> MSSDLAAELGFDPALKKKKKTKKVIPDDFDAAVNGKENGSGDDLFAGLKKKKKKSKSVSADAEAEKEPTDDIAEALGELSLKKKKKKTKDSSVDAFEKELAKAGLDNVDAESKEGTPSANSSIQQEVGLPYSELLSRFFNILRTNNPELAGDRSGPKFRIPPPVCLRDGKKTIFSNIQDIAEKLHRSPEHLIQYLFAELGTSGSVDGQKRLVIKGKFQSKQMENVLRRYILEYVTCKTCKS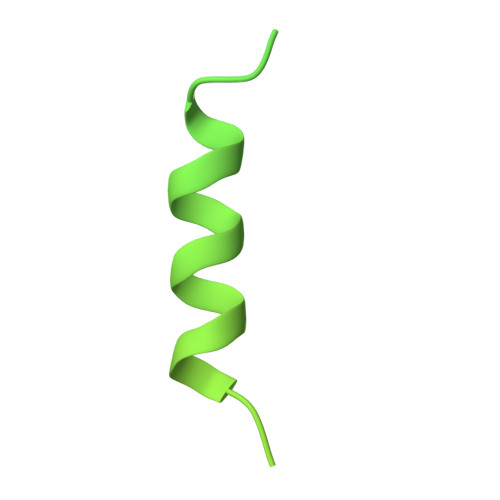INTELKREQSNRLFFMVCKSCGSTRSVSSIKTGFQATVGKRRRM> GPDFSKHLKEETIQIITKASHEHEDKSPETVLQSAIKLEYARLVKLAQEDTPPETDYRLHHVVVYFIQNQAPKKIIEKTLLEQFGDRNLSFDERCHNIMKVAQAKLEMI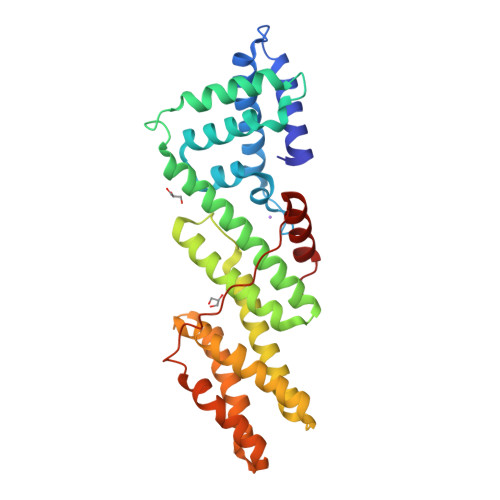KPEEVNLEEYEEWHQDYRKFRETTMYLIIGLENFQRESYIDSLLFLICAYQNNKELLSKGLYRGHDEELISHYRRECLLKLNEQAAELFESGEDREVNNGLIIMNEFIVPFLPLLLVDEMEEKDILAVEDMRNRWCSYLGQEMEPHLQEKLTDFLPKLLDCSMEIKSFHEPPKLPSYSTHELCERFARIMLSLS> GSGSPLAQQI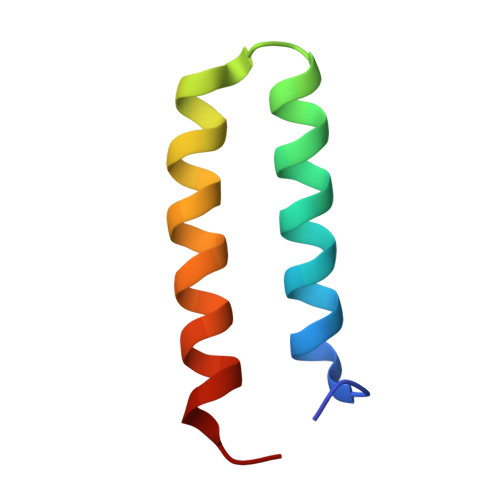KNIHSFIHQAKAAGRMDEVRTLQENLHQLMHEYFQQSD>[3x]GPQDPDKRRKTLVIIEKTYSLLLDVEDYERRYLLSLEEERPALMDDRKHKICSMYDNLRGKLPGQERPSDDHFVQIMC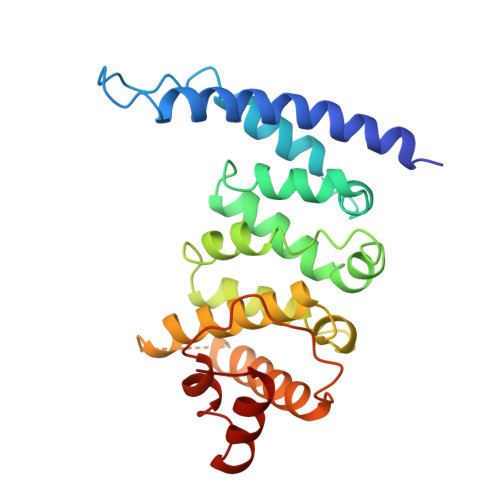IRKGKRMVARILPFLSTEQAADILMTTARNLPFLIKKDAQDEVLPCLLSPFSLLLYHLPSVSITSLLRQLMNLPGSPHLTAVLQNKFGLSLLLILLSRGEDLQSSDPATESTQNNQWTEVMFMATRELLRIPQAALAKPISIPTNLVSLFSRYVDRQKLNLLETKLQLVQ>MDKERIIQEFVPGKQVTLAHLIAHPGEELAKKIGVPDAVAIGIMTLTPGETAMIAGDLALKAADVHIGFLDRFSGALVIYGSVGAVEEALSQTVSGLGRLLNYTLCEMTKSLEHHHHHH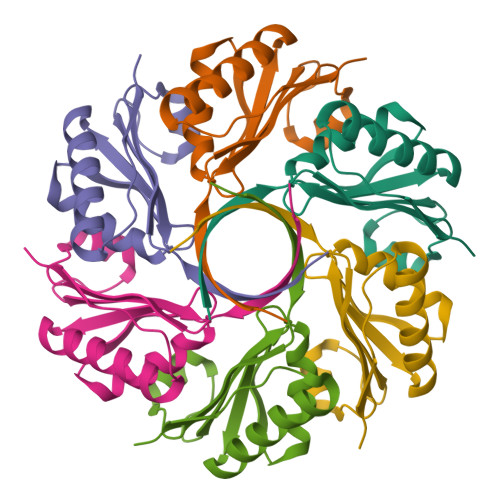[48x]> MGTGKELVLAL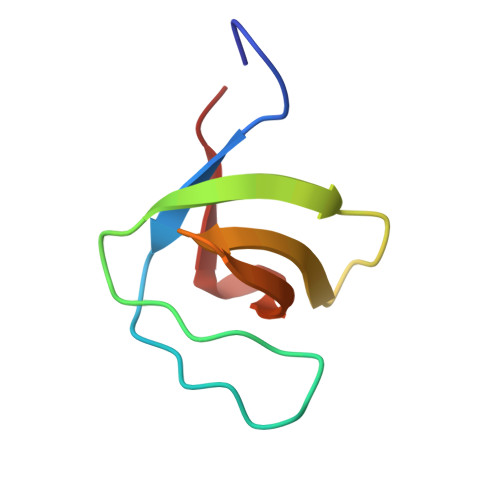YDYQEKSPREVTMKKGDILTLLNSTNKDWWKVEVNDRQGFVPAAYVKKLD> MTTPPVVANYENASMAADYIKRVSNVLPDIGIICGSGLGKLIEEIEERKVIPYINIPNFPKTTVAGHVGNLVLGSVGGRKIVAMQGRLHMYEGYSNQEIALPIRVMKLLGVRVLLITNLAGGINRKLKSGDFVLIKGHINFPGLGLNNVLVGPNQDEFGPRFPDLSNAYDRLLQQLALKIAQENDFQDLVHEGVYAFNGGPTYESPDESNMLLKLGCDVVGMSTVPEVIIACHCGIKVLAVSLIANNSILDAENDVSINHEKVLAVAEKRADLLQMWFKEIITRLPLD

Purine nucleoside phosphorylase (PNP) (E.C 2.4.2.1) is an enzyme responsible for reversible phosphorolysis of purine nucleosides, generating ribose-1-phosphate and their corresponding bases. Here, we characterize a newly identified isoform of S. mansoni PNP (SmPNP2) employing a combination of methodologies: ligand discovery by thermofluorescence, kinetic assays, high-performance liquid chromatography (HPLC) and X-ray crystallography. The crystal structure reveals this property appears to be related to the substitutions in the active site that induce the locking of the gate loop.

Structural information of SmPNP2 in both the apo form and in complexes with cytidine, cytosine, ribose-1-phosphate, adenine, hypoxanthine, and tubercidin was obtained. SmPNP2 was readily crystallized in several conditions, ranging from pH 4.0 to pH 9.0, in cubic space group P213 with one monomer per asymmetric unit. The main difference between the SmPNP1 and SmPNP2 structures is the presence of α-helix formed by residues 247–252 in the latter, at the beginning of the gate loop (residues 244–260). The presence of an Ala118Leu substitution results in conformational changes of the phosphate loop centered on the Ser35 residue. The presence of a bulkier leucine group in place of alanine next to the Ser35 residue in SmPNP2 blocks the movement necessary to assume a closed conformation due to steric hindrance maintaining this loop permanently in an open conformation. The presence of a new α-helix formed by residues 247–252 and the substitution Ala118Leu also appear to have a large impact in the active site and gate loop conformations. This can be seen by calculating the RMSD of Cαs of residues 244–247, which display a values 2.84 Å, thus indicating a considerable deviation from the structure of SmPNP1.The linear ubiquitin (Ub) chain assembly complex (LUBAC) generates Met1-linked “linear” Ub chains that regulate the activation of the nuclear factor κB (NFκB) transcription factor and other processes. (2006) identified the linear Ub chain assembly complex (LUBAC), which consists of the chain-assembling E3 ligase HOIP as well as HOIL-1 and SHARPIN (Walczak et al., 2012). HOIP also comprises several NPL4 zinc finger (NZF) Ub binding domains (UBDs) that target it to ubiquitinated proteins (Haas et al., 2009), a Ub-associated (UBA) domain that mediates interactions with HOIL-1 (Yagi et al., 2012), and N-terminal PUB (peptide:N-glycanase/UBA- or UBX-containing proteins) and B box domains of unknown functions. Here, we show that OTULIN interacts directly with the N-terminal PUB domain of HOIP via a conserved PUB-interacting motif (PIM) in OTULIN.

Our structure contains 13 molecules within the asymmetric unit that superimpose with a low root-mean-square deviation (rmsd; 0.9–1.2 Å). As anticipated, residues 59–158 of HOIP form a PUB domain resembling that of PNGase, the only other PUB domain structurally characterized to date (Allen et al., 2006; Zhao et al., 2007). HOIP and PNGase superimpose with an rmsd of 7.2 Å for residues 59–158 of HOIP, and most secondary structure elements are conserved. In addition, the HOIP PUB domain contains two N-terminal helices and one C-terminal helix that contribute to the hydrophobic core of the PUB domain, revealing why shorter constructs were insoluble. Hydrophobic residues within the N-terminal extension are conserved among most HOIP orthologs, suggesting that the extended fold is conserved. In contrast, the residues forming a putative PIM pocket are highly conserved in HOIP. The HOIP PIM pocket is formed by hydrophobic residues located on helices α4 (equivalent to helix α2 in PNGase, hereafter named αA) and α5 (equivalent to helix α3 in PNGase, hereafter named αB) and on the β1 strand (compare Figures 2B and 1E). In our apo structures, the side chain of Tyr94 is rotated to bind the HOIP Tyr pocket in cis, appearing to block access to the PIM pocket.

>[13x]GPMPGEEEERAFLVAREELASALRRDSGQAFSLEQLRPLLASSLPLAARYLQLDAARLVRCNAHGEPRNYLNTLSTALNILEKYGRNLLSPQRPRYWRGVKFNNPVFRSTVDAVQGGRDVLRLYGYTEEQPDGLSFPEGQEEPDEHQVATVTLEVLLLRTELSLLLQNTHPRQQALEQLLEDKVED> GTRSESTEGHSKDLLYKYKLYGDIDEYAYYFLDIDIGTPEQRISLILDTGSSSLSFPCAGCKNCGVHMENPFNLNNSKTSSILYCENEECPFKLNCVKGKCEYMQSYCEGSQISGFYFSDVVSVVSYNNERVTFRKLMGCHMHEESLFLYQQATGVLGMSLSKPQGIPTFVNLLFDNAPQLKQVFTICISENGGELIAGGYDPAYIVRRGGSKSVSGQGSGPVSESLSESGEDPQVALREAEKVVWENVTRKYYYYIKVRGLDMFGTNMMSSSKGLEMLVDSGSTFTHIPEDLYNKLNYFFDILCIQDMNNAYDVNKRLKMTNESFNNPLVQFDDFRKSLKSIIAKENMCVKIVDGVQCWKYLEGLPDLFVTLSNNYKMKWQPHSYLYKKESFWCKGIEKQVNNKPILGLTFFKNRQVIFDIQKNRIGFVDANCPSHPTHTRPRLENLYFQGDYKDDDDKH

A library of known aspartic protease inhibitors was screened to identify compounds that inhibit plasmepsin V from Plasmodium vivax. This screen revealed compounds with an imino‐pyrimidinone‐fused pyrrolidine (IPF) scaffold that exhibited sub‐micromolar inhibitory activity against plasmepsin V. Further screening of IPF analogs against the related aspartic protease plasmepsin X showed inhibitory activity, while a third aspartic protease, plasmepsin IX, was not significantly inhibited.

Modifications to the P1 biaryl region of the IPF scaffold differentially modulated inhibition of both plasmepsin V and X. Notably, analogs with potent plasmepsin X inhibitory activity successfully blocked the growth of Plasmodium falciparum in vitro. X‐ray structures of IPF analogs in complex with plasmepsin V provided insights into their binding mode and revealed avenues to further improve IPF potency and selectivity between plasmepsin V and X. This understanding of how these compounds interact with the active sites of plasmepsin V and X will serve as a foundation for the future design of dual inhibitors targeting these proteases.(3~{R})-1-ethanoylpyrrolidine-3-carboxylic acid | C7 H11 N 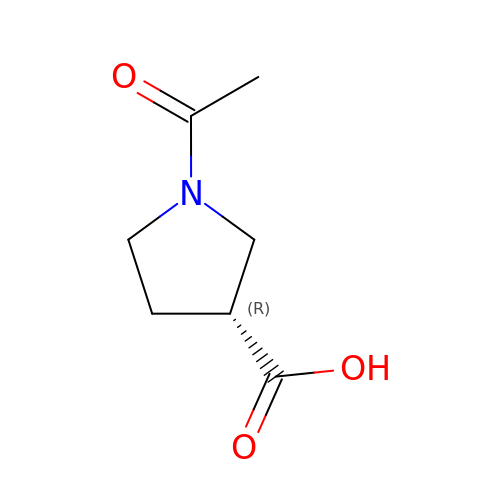O3 | FEQQMBBBBFVNMN-ZCFIWIBFSA-N>[4x]GSGSHVTLPFYPKSPQSKDLIKEAILDNDFMKNLELSQIQEIVDCMYPVEYGKDSCIIKEGDVGSLVYV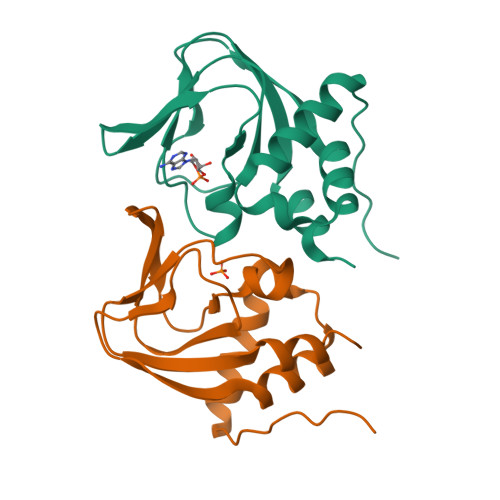MEDGKVEVTKEGVKLCTMGPGKVFGELAILYNCTRTATVKTLVNVKLWAIDRQCFQTIMMRTGLIKHTEY> MSTATARRRVVLTGFGVISSIGTGVEEYTAGLRAGRSGARPITRFDTEGFGQNTACEVPDFEPGRWIHHVPLDDMGRAGQYAVAAARMAVDDAGLTEDDLGERQAVITVGTTDGESHDIAVLLEQELAAGDPEAMDPVLARRINAGRLSTVIARELRMPNVEATTVTTACAAGNYSVGYGLDSIRSGEVDIALCGGADAVCRKAFALFKRFGALTPDVVRPFDKDRQGILTGEGAGILVLESLESALARGARIHAEVLGYGLSCDAAHPTAPNRDGIARGIRLALDDAGVEQEEIDFISAHGTGTKANDKTESAAIVDVYGDAPPRTVAVKSMLGHSMGAASALGAIACGLAIEHGF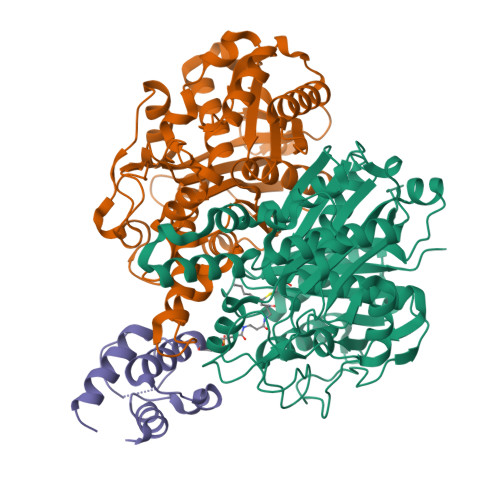IPPTINHRETDPDCPLDVVPNRAVEADVRIVQNNSSAFAGNNAVLILGTYGE;> MTTMSTATARPEATLPPGTPVITGWSAVSPYGIGRAEFAAGVRAGAKTAVKADAGLGPLPSSDVCTVPGFDIQEQLGPRGTAKMDRLTALALVASDGLLLDADGNRAVATDELTGVVLGITMGSLENVTDFLRQSYTNARPFYVDAGRIPFGSLNHAAGATAIRHDLKGPNTTVAGGRVSGLLALNYARRLMGQGRATKYLVGSAEEFSAAHAWFEHTATASGDPAPLLGEGCGLFLVEQAEAAERPPLAAVLSVETRVDIDDDPGAAVTACARRALRRAGVDAGEVWAAVPCAAPTAAGRAEHEALAALVPADALSRVPSMELLGDTGAASASFQIAAVLAAAEADADSRGRIALVCAVDRDGAVAVAVLRLIGEQR;> MTTVAPERLSRIREIIAENIDVDLDGLSDTALFIDELGADSLKLIDVLSALEMEYSIVIDMNELPKMTNVEATYQVTAAAAGW>MTQDELKKAVGWAALQYVQPGTIVGVGTGSTAAHFIDALGTMKG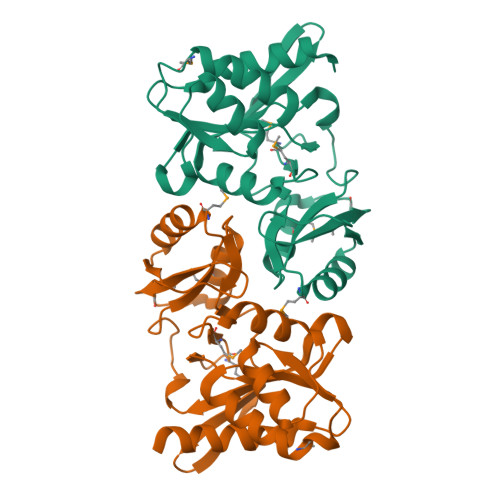QIEGAVSSSDASTEKLKSLGIHVFDLNEVDSLGIYVDGADEINGHMQMIKGGGAALTREKIIASVAEKFICIADASKQVDILGKFPLPVEVIPMARSAVARQLVKLGGRPEYRQGVVTDNGNVILDVHGMEILDPIAMENAINAIPGVVTVGLFANRGADVALIGTPDGVKTIVK[2x]(2R)-7-[(2R,3R,4R,5S,6S)-6-(hydroxymethyl)-3-[(2R,3R,4R,5R,6S)-6-methyl-3,4,5-tris(oxidanyl)oxan-2-yl]oxy-4,5-bis(oxidanyl)oxan-2-yl]oxy-2-(4-methoxy-3-oxidanyl-phenyl)-5-oxidanyl-2,3-dihydrochromen-4-one | C28 H34 O15 | 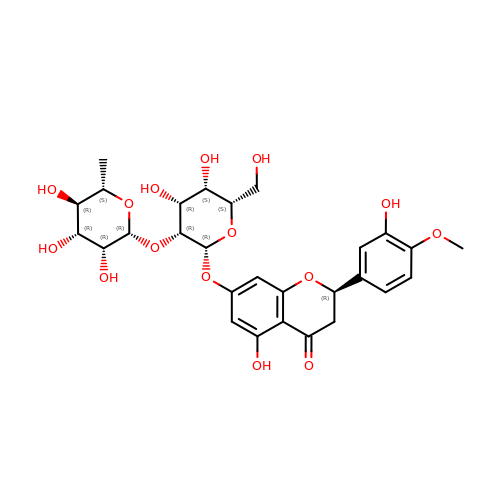ARGKVCXINMKCAZ-LIVPLLNOSA-N> MAAVDIRDNLLGISWVDSSWIPILNSGSVLDYFSERSNPFYDRTCNNEVVKMQRLTLEHLNQMVGIEYILLHAQEPILFIIRKQQRQSPAQVIPLADYYIIAGVIYQAPDLGSVINSRVLTAVHGIQSAFDEAMSYCR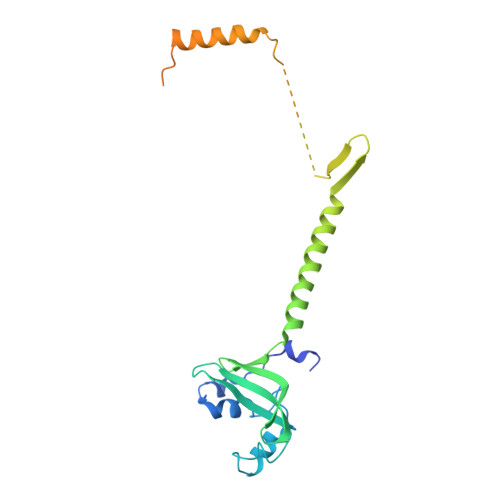YHPSKGYWWHFKDHEEQDKVRPKAKRKEEPSSIFQRQRVDALLLDLRQKFPPKFVQLKPGEKPVPVDQTKKEAEPIPETVKPEEKETTKNVQQTVSAKGPPEKRMRLQ>MAFKVISQENLLEQKRKETLQEDIPFIVNGEMEYVTKKISNGEMETLELNKPLGEMMTFSSTSNLKELLRKVVLDVELGREQVQLLYKPIYDSIADSNLPQVMDAKWALQGNCVFLEHIEGEEIKFGTINAENGPVARIQTYATGFEYTKEMKDFNQTFSVEILNKSIGESYNALLNHIHLSPIINFNYKASNKTAFKGETNDPIWLGIWRTLTQAQKDTVIAKRQGNILMASSADQIEIEMALNGGHLLNGSMYPSIKNISTVIYYDGWEVTVGKKTYSYKGVTPGKGYLIRPKRGFKELIKRDLTTEVGNADLSKLVENQIVGHCYRGAFAAVEENVQEISFR[10x];>MAFKGQPTPSTITQITRAKISDGKSVRVILSEGESTKTQQFYLINGFFGVAMQDGEKGDEVTLQIEQAEYETDNIVTSEAFEAGKLIYWDNTAKKFTTTSASNRLVGRVTDGKDSNNVIWFILLPQQ[15x]

Here, we reveal the extended and contracted atomic structures of an intact contractile-tailed phage (φCD508) that binds to and penetrates the protective S-layer of the Gram-positive human pathogen Clostridioides difficile. The virion can be divided into five distinct regions: the head, neck, tail, baseplate, and needle. Structures of purified φCD508 virions in both extended and contracted conformations were determined by single-particle EM of frozen-hydrated samples; the resolution ranged from 2.6 to 4.0 Å for the extended phage, and 2.9 to 4.2 Å for the contracted form.

At the base of the capsid sits a unique opening, centered on what would be a fivefold symmetry axis in a complete icosahedron; it is made up of 12 copies of portal protein gp45, forming an opening through which DNA is ejected from the capsid. Thus, there is a 5–12-fold symmetry mismatch between the capsid and the portal. (K) CryoEM density of C1 portal/capsid assembly showing the symmetry mismatch between gp48 capsid decoration trimers and the dodecameric portal assembly. Inset shows lacking density for the N-terminal arm of one portal-proximal gp48 protein.>[5x]PVVIKTEGPAWTPLEPKLITRLADTVRTKGLRSPITMAEVEALMSSPLLPHDVTNLMRVILGPAPYALWMDAWGVQLQTVIAAATRDPRHPANGQGRGERT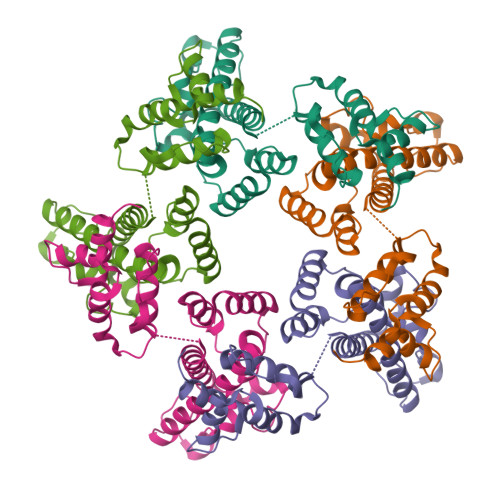NLNRLKGLADGMVGNPQGQAALLRPGELVAITASALQAFREVARLAEPAGPWADIMQGPSESFVDFANRLIKAVEGSDLPPSARAPVIIDCFRQKSQPDIQQLIRTAPSTLTTPGEIIKYVLDRQKTA>[2x]MAHHHHHHMTQSVCILGVTGSIGRSTLKILGQHPDKYSVFAVSAHSRISELVEICKQFRPKVVVVPEQKIAELKTLFAQQNISDIDVLAGQEGLVDIASHTDVDIVMAAIVGAAGLLPTLAAVKAGKRVLLANKEALVMSGEIMMQAARDHQALLLPVDSEHNAIFQSLPHNYLQADRTG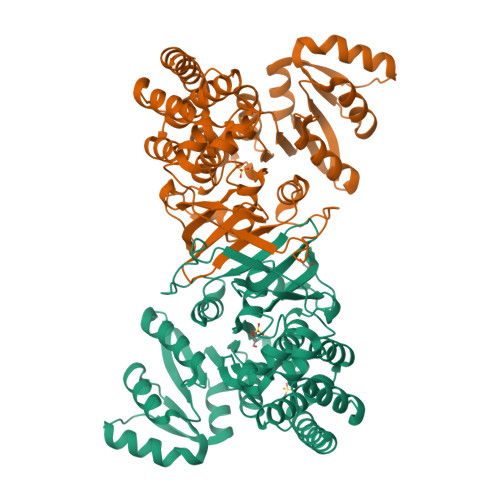QPQLGVSKILLTASGGPFLNHSLEQLVHVTPQQACKHPNWSMGQKISVDSATLMNKGLELIEACHLFSISEHFVTVVVHPQSIIHSMVQYVDGSTLAQMGNPDMCTPIAHALAWPERLQTNVPALDLFEYSQLNFQAPDTQKFPALNLARQAMRAGGLAPTILNAANEIAVEAFLMERIGFTSIPQVVEHTLEKLENAAAESIECILDKDKVARSVAQQYISSIGG> GAMGSMETFDPTELPELLKLYYRRLFPYSQYYRWLNYGGVIKNYFQHREFSFTLKDDIYIRYQSFNNQSDLEKEMQKMNPYKIDIGAVYSHRPNQHNTVKLGAFQAQEKELVFDIDMTDYDDVRRCCSSADICPKCWTLMTMAIRIIDRALKEDFGFKHRLWVY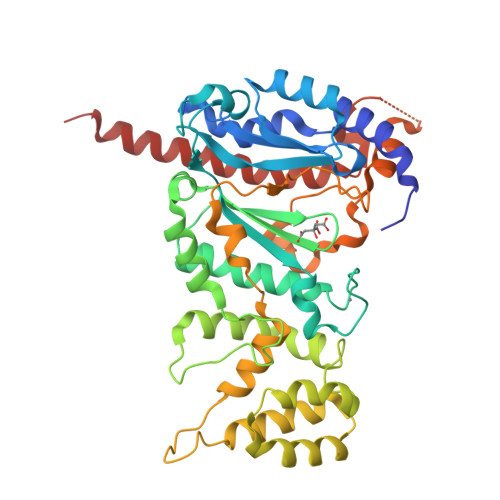SGRRGVHCWVCDESVRKLSSAVRSGIVEYLSLVKGGQDVKKKVHLSEKIHPFIRKSINIIKKYFEEYALVNQDILENKESWDKILALVPETIHDELQQSFQKSHNSLQRWEHLKKVASRYQNNIKNDKYGPWLEWEIMLQYCFPRLDINVSKGINHLLKSPFSVHPKTGRISVPIDLQKVDQFDPFTVPTISFICRELDAISTNEEEKEENEAESDVKHRTRDYKKTSLAPYVKVFEHFLENLDKSRKGELLKKSDLQKDF> GSPEGVPICGACR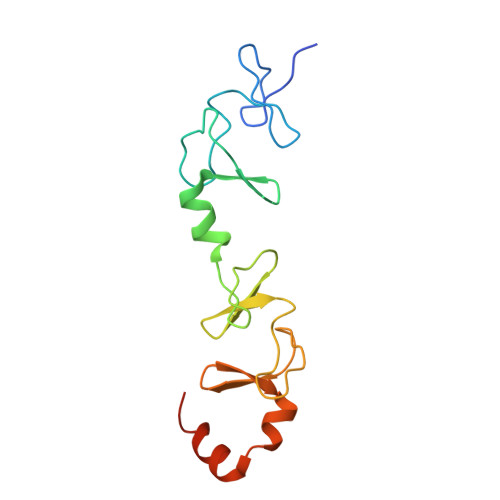RPIEGRVVNAMGKQWHVEHFVCAKCEKPFLGHRHYERKGLAYCETHYNQLFGDVCFHCNRVIEGDVVSALNKAWCVNCFACSTCNTKLTLKNKFVEFDMKPVCKKCYEKFPLELKKRLKKLAETLGRK>[4x]MRTISFFNNKGGVGKTTLSTNVAHYFALQGKRVLYVDCDPQCNATQLMLTEEQTESIYLDGLNDEVAERNSLAKTVYAIFVPLREGESQIAAEITPMRSERFGVDVLPGHPALSQIEDLMSDSWQSALGRQTGPFRRIHWAGQLAHAMERDDRYDVIFFDVGPSLGPFNRTVLLGCDAFVTPTATDLFSFHAFG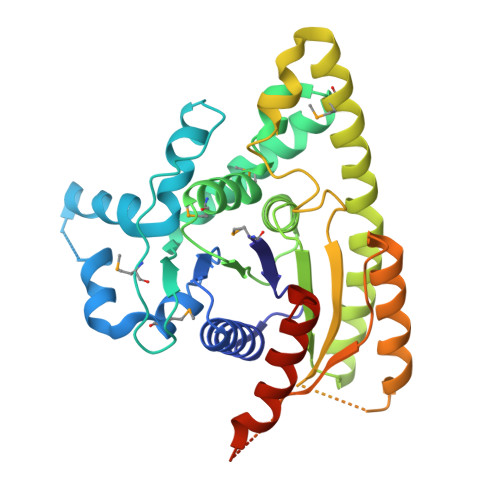NLARWFDAWVTQYAEIHEGNMAEWKKYSADVEAKTRPLRLGGFDGEGLRYLGYTTLEYVKRRANGQEQLVGAFERFRGRFAAEAERISNSLSKHSNSTLLGHVPHMHSMPATAQDVHAPIMELSSSDRVRGAQINQRNAYAEKINSVAANVYKALFPNELEHHHHHH> MFGSGNVLPVKIQPPLLRPLAYRVLSRKYGLSIKSDGLSALAEFVGTNIGANWRQGPATIKFLEQFAAVWKQQERGLFIDQSGVKEVIQEMKEREKVEWSHEHPIQHEENILGRTDDDENNSDDEMPIAADSSLQNVSLSSPMRQPTERDEYKQPFKPESSKALDWRDYFKVINASQQQRFSYNPHKMQFIFVPNKKQNGLGGIAGFLPDIEDKVQMFLTRYYLTNDRVMRNENFQNSDMFNPLSSMVSLQNELSNTNRQQQSSSMSITPIKNLLGRDAQNFLLLGLLNKNFKGNWSLEDPSGSVEIDISQTIPTQGHYYVPGCMVLVEGIYYSVGNKFHVTSMTLPPGERREITLETIGNLDLLGIHGISNNNFIARLDKDLKIRLHLLEKELTDHKFVILGANLFLDDLKIMTALSKILQKLNDDPPTLLIWQGSFTSVPVFASMSSRNISSSTQFKNNFDALATLLSRFDNLTENTTMIFIPGPNDLWGSMVSLGASGTLPQDPIPSAFTKKINKVCKNVVWSSNPTRIAYLSQEIVIFRDDLSGRFKRHRLEFPFNESEDVYTENDNMMSKDTDIVPIDELVKEPDQLPQKVQETRKLVKTILDQGHLSPFLDSLRPISWDLDHTLTLCPIPSTMVLCDTTSAQFDLTYNGCKVINPGSFIHNRRARYMEYVPSSKKTIQEEIYI;> MSNLVKEKAPVFPISKVKKIAKCDPEYVITSNVAISATAFAAELFVQNLVEESLVLAQLNSKGKTSLRLSLNSIEECVEKRDNFRFLEDAIKQLKKNSALDKKRELNMQPGRSDQEVVIEEPELHEDDGVEEEEEEDEVSEEEEPVHNEELLDDSKDQQNDKSTRSVASLLSRFQYKSALDVGEHSDSSDIEVDHTKSTDP;> MPPKGWRKDAQGNYPTTSYIKEQENITIQDLLFPKSTIVNLAREVPQQSGKKLLINKDASLALQRGATVFVNHLLLFAREIAKSQDKKSCSVDDVLSALDHIGHSALKGPVRDKLDEYQAAVEQRKKEKLDSGEVDADGDIDMGEDKENVPVEKVKEHDEIEEQGDALQDVEESSEKKQKTESQDVETRVQNLEQT;> MMFGKKKNNGGSSTARYSAGNKYNTLSNNYALSAQQLLNASKIDDIDSMMGFERYVPPQYNGRFDAKDIDQIPGRVGWLTNMHATLVSQETLSSGSNGGGNSNDGERVTTNQGISGVDFYFLDEEGGSFKSTVVYDPYFFIACNDESRVNDVEELVKKYLESCLKSLQIIRKEDLTMDNHLLGLQKTLIKLSFVNSNQLFEARKLLRPILQDNANNNVQRNIYNVAANGSEKVDAKHLIEDIREYDVPYHVRVSIDKDIRVGKWYKVTQQGFIEDTRKIAFADPVVMAFDIETTKPPLKFPDSAVDQIMMISYMIDGEGFLITNREIISEDIEDFEYTPKPEYPGFFTIFNENDEVALLQRFFEHIRDVRPTVISTFNGDFFDWPFIHNRSKIHGLDMFDEIGFAPDAEGEYKSSYCSHMDCFRWVKRDSYLPQGSQGLKAVTQSKLGYNPIELDPELMTPYAFEKPQHLSEYSVSDAVATYYLYMKYVHPFIFSLCTIIPLNPDETLRKGTGTLCEMLLMVQAYQHNILLPNKHTDPIERFYDGHLLESETYVGGHVESLEAGVFRSDLKNEFKIDPSAIDELLQELPEALKFSVEVENKSSVDKVTNFEEIKNQITQKLLELKENNIRNELPLIYHVDVASMYPNIMTTNRLQPDSIKAERDCASCDFNRPGKTCARKLKWAWRGEFFPSKMDEYNMIKRALQNETFPNKNKFSKKKVLTFDELSYADQVIHIKKRLTEYSRKVYHRVKVSEIVEREAIVCQRENPFYVDTVKSFRDRRYEFKGLAKTWKGNLSKIDPSDKHARDEAKKMIVLYDSLQLAHKVILNSFYGYVMRKGSRWYSMEMAGITCLTGATIIQMARALVERVGRPLELDTDGIWCILPKSFPETYFFTLENGKKLYLSYPCSMLNYRVHQKFTNHQYQELKDPLNYIYETHSENTIFFEVDGPYKAMILPSSKEEGKGIKKRYAVFNEDGSLAELKGFELKRRGELQLIKNFQSDIFKVFLEGDTLEGCYSAVASVCNRWLDVLDSHGLMLEDEDLVSLICENRSMSKTLKEYEGQKSTSITTARRLGDFLGEDMVKDKGLQCKYIISSKPFNAPVTERAIPVAIFSADIPIKRSFLRRWTLDPSLEDLDIRTIIDWGYYRERLGSAIQKIITIPAALQGVSNPVPRVEHPDWLKRKIATKEDKFKQTSLTKFFSKTKNVPTMGKIKDIEDLFEPTVEEDNAKIKIARTTKKKAVSKRKRNQLTNEEDPLVLPSEIPSMDEDYVGWLNYQKIKWKIQARDRKRRDQLFGNTNSSRERSALGSMIRKQAESYANSTWEVLQYKDSGEPGVLEVFVTINGKVQNITFHIPKTIYMKFKSQTMPLQKIKNCLIEKSSASLPNNPKTSNPAGGQLFKITLPESVFLEEKENCTSIFNDENVLGVFEGTITPHQRAIMDLGASVTFRSKAMGALGKGIQQGFEMKDLSMAENERYLSGFSMDIGYLLHFPTSIGYEFFSLFKSWGDTITILVLKPSNQAQEINASSLGQIYKQMFEKKKGKIETYSYLVDIKEDINFEFVYFTDISKLYRRLSQETTKLKEERGLQFLLLLQSPFITKLLGTIRLLNQMPIVKLSLNEVLLPQLNWQPTLLKKLVNHVLSSGSWISHLIKLSQYSNIPICNLRLDSMDYIIDVLYARKLKKENIVLWWNEKAPLPDHGGIQNDFDLNTSWIMNDSEFPKINNSGVYDNVVLDVGVDNLTVNTILTSALINDAEGSDLVNNNMGIDDKDAVINSPSEFVHDA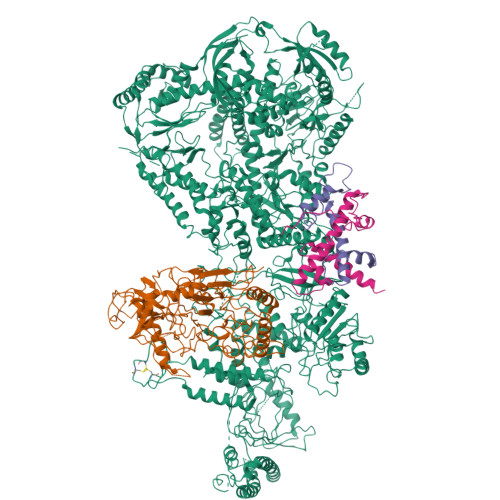FSNDALNVLRGMLKEWWDEALKENSTADLLVNSLASWVQNPNAKLFDGLLRYHVHNLTKKALLQLVNEFSALGSTIVYADRNQILIKTNKYSPENCYAYSQYMMKAVRTNPMFSYLDLNIKRYWDLLIWMDKFNFSGLACIEIEEKENQDYTAVSQWQLKKFLSPIYQPEFEDWMMIILDSMLKTKQSYLKLNSGTQRPTQIVNVKKQDKEDSVENSLNGFSHLFSKPLMKRVKKLFKNQQEFILDPQYEADYVIPVLPGSHLNVKNPLLELVKSLCHVMLLSKSTILEIRTLRKELLKIFELREFAKVAEFKDPSLSLVVPDFLCEYCFFISDIDFCKAAPESIFSCVRCHKAFNQVLLQEHLIQKLRSDIESYLIQDLRCSRCHKVKRDYMSAHCPCAGAWEGTLPRESIVQKLNVFKQVAKYYGFDILLSCIADLTI4-(2-methyl-3-propan-2-yl-imidazol-4-yl)-~{N}-(4-methylsulfonylphenyl)pyrimidin-2-amine | C18 H21 N5 O2 S | 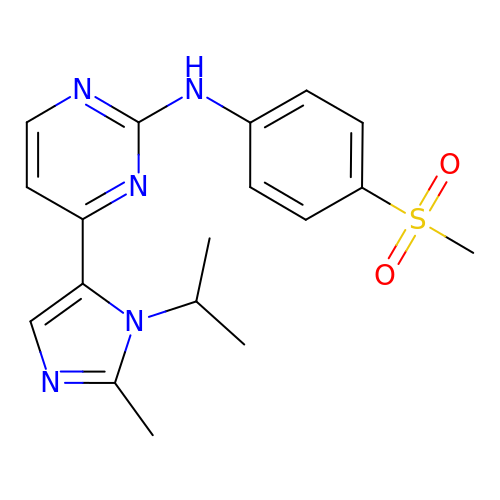WJRRGYBTGDJBFX-UHFFFAOYSA-N> GSMAAQRRSLLQSEQQPSWTDDLPLCHLSGVGSASNRSYSADGKGTESHPPEDSWLKFRSENNCFLYGVFNGYDGNRVTNFVAQRLSAELLLGQLNAEHAEADVRRVLLQAFDVVERSFLESIDDALAEKASLQSQLPEGVPQHQLP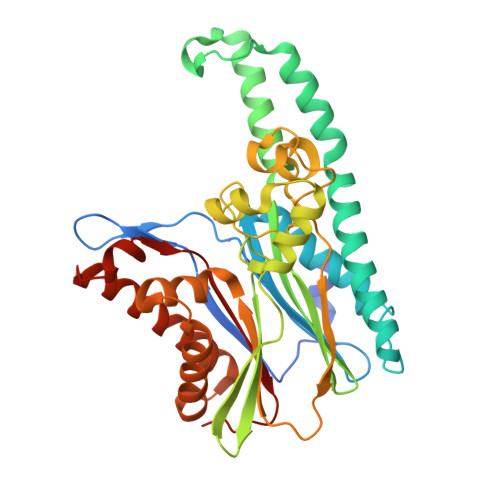PQYQKILERLKTLEREISGGAMAVVAVLLNNKLYVANVGTNRALLCKSTVDGLQVTQLNVDHTTENEDELFRLSQLGLDAGKIKQVGIICGQESTRRIGDYKVKYGYTDIDLLSAAKSKPIIAEPEIHGAQPLDGVTGFLVLMSEGLYKALEAAHGPGQANQEIAAMIDTEFAKQTSLDAVAQAVVDRVKRIHSDTFASGGERARFCPRHEDMTLLVRNFGYPLG>[2x]MDHHHHHHHHMPRTTGMNVAVVGGGISGLAVAHHLRSRGTDAVLLESSARLGGAVGTHALAGYLVEQGPNSFLDREPATRALAAALNLEGRIRAADPAAKRRYVYTRGRLRSVPASPPAFLASDILPLGARLRVAGELFSRRAPEGVDESLAAFGRRHLGHRATQVLLDAVQTGIYAGDVEQLSVAATFPMLVKMEREHRSLILGAIRAQKAQRQAALPAGTAPKLSGALSTFDGGLQVLIDA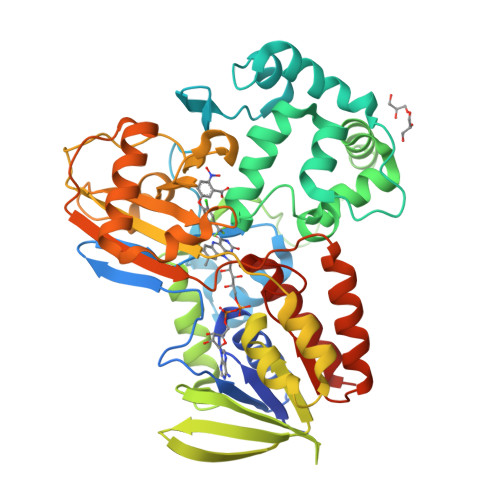LAASLGDAAHVGARVEGLAREDGGWRLIIEEHGRRAELSVAQVVLAAPAHATAKLLRPLDDALAALVAGIAYAPIAVVHLGFDAGTLPAPDGFGFLVPAEEQRRMLGAIHASTTFPFRAEGGRVLYSCMVGGARQPGLVEQDEDALAALAREELKALAGVTARPSFTRVFRWPLGIPQYNLGHLERVAAIDAALQRLPGLHLIGNAYKGVGLNDCIRNAAQLADALVAGNTSHAP> ADYQGKNVVIIGLGLTGLSCVDFFLARGVTPRVMDTRMTPPGLDKLPEAVERHTGSLNDEWLMAADLIVASPGIALAHPSLSAAADAGIEIVGDIELFCREAQAPIVAITGSNGKSTVTTLVGEMAKAAGVNVGVGGNIGLPALMLLDDECELYVLELSSFQLETTSSLQAVAATILNVTEDHMDRYPFGLQQYRAAKLRIYENAKVCVVNADDALTMPIRGADERCVSFGVNMGDYHLNHQQGETWLRVKGEKVLNVKEMKLSGQHNYTNALAALALADAAGLPRASSLKALTTFTGLPHRFEVVLEHNGVRWINDSKATNVGSTEAALNGLHVDGTLHLLLGGDGKSADFSPLARYLNGDNVRLYCFGRDGAQLAALRPEVAEQTETMEQAMRLLAPRVQPGDMVLLSPACASLDQFKNFEQRGNEFARLAKELGS

MurD catalyzes the addition of D-glutamic acid to UDP-MurNAc-L-Ala, generating the dipeptide moiety L-Ala-D-Glu in almost all bacterial species. From a structural point of view, Mur ligases are three-domain enzymes that share a very well conserved ATP-binding site that harbors the Gly-X-X-Gly-Lys-Thr/Ser motif and display notable structural similarities in terms of domain arrangement. The N-terminal domain is involved in the binding of the UDP-precursor, the central domain in the binding of ATP, and the C-terminal domain in the binding of the amino acid or dipeptide. Crystal structures of Mur ligases reveal that MurC, MurD and MurF display at least two distinct conformations, namely ‘open’ and ‘closed’, with the position of C-terminal domain dictating the nature of the conformation.

Intermediate Bound MurD was co-crystallized with UMA and AMP-PNP in order to further explore the dynamics of MurD upon ligand binding. During the process of structure solution, 423 residues were refined. Structural inspection of Intermediate Bound MurD revealed that Lys198 is not carbamoylated, contrary to all previously published structures of MurD complexed to UMA Previously, complex formation between MurD and UMA, UDP-N-acetylmuramoyl-L-alanyl-D-glutamic acid (UMAG), UMA-ADP, UMA-ADP-Mg2+ and UMA-ADP-Mn2+ locked MurD in a closed structure, which gave weight to the proposal that ligand binding was important for the movement of the C-terminal domain leading to closure. It appeared that it was not in a closed conformation. After superposition of Intermediate Bound MurD with open UMA-bound MurD, we confirmed that this new conformation of MurD is different from the previously described ones, which was quantified by the determination of the RMSD values of all of the superimposed structures, both for the whole protein and for distinct domains. In the Intermediate Bound MurD structure, the H-bond pattern of UMA binding is almost the same as in the closed structures of MurD and as in open UMA-bound MurD. ADP-binding residues also occupy the same orientations as in previously solved structures. When focusing on the interactions and position of Arg302 in Intermediate Bound MurD, we observed a novel H-bond pattern for Arg302. Intermediate Bound MurD displays some features of the closed conformation of MurD. The hinge loop is similar to the one in open conformation of MurD, but with an additional H-bond to Pro300 and ADP, thus dictating the C-terminal domain to take a position closer to central domain than open conformation of MurD. However, the C-terminal domain does not rotate to the closed conformation, because Arg302 is not H-bonded to Leu299 as it is the case in closed MurD.>ACCGGCCGG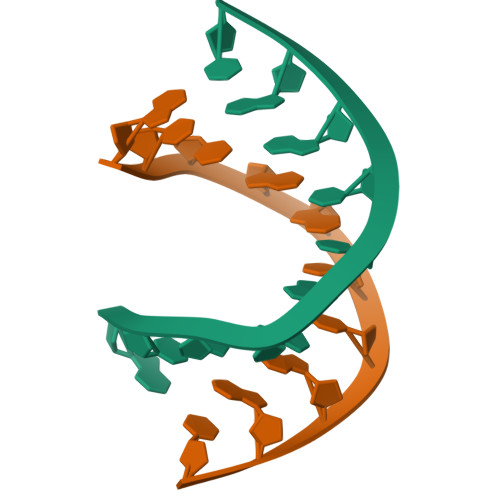T[2x]>[6x]MSPIHVRAHPGDVAERVLLPGDPGRAEWIAKTFLQNPRRYNDHRGLWGYTGLYKGV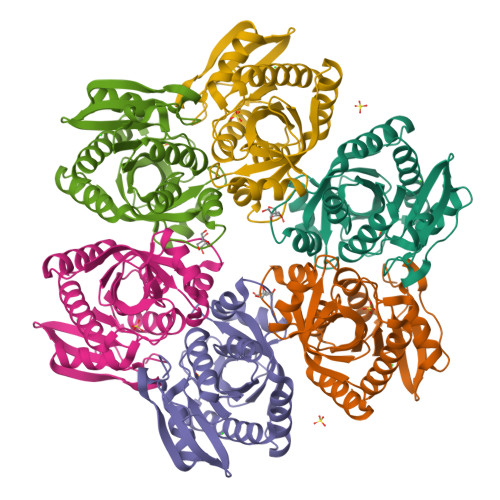PVSVQTTGMGTPSAAIVVEELVRLGARVLVRVGTAGAASSDLAPGELIVAQGAVPLDGTTRQYLEGRPYAPVPDPEVFRALWRRAEALGYPHRVGLVASEDAFYATTPEEARAWARYGVLAFEMEASALFLLGRMRGVRTGAILAVSNRIGDPELAPPEVLQEGVRRMVEVALEAVLEV> LFRAL;> AKCVSYGVAQIKAPALHSQGYTGSNVKVAILGTGIDSSHPDLNVAGGASFVPSETNPFQDNSSHGTHIAGTVLAVAPSASLYAVKVLGADGSGQASWVINGIEWAIANNMDVINMSLGSPSGSAALKAAVDKAVASGVVVVAAAGNSGTSGSSSTVTYPAKYPSVIAVGAVDSSNQRAPFSSVGPELDVMAPGVSICSTLPGGKYGALSGTSMASPHVAGAAALILSKHPNWTNTQVRSSLENTATKLGDSFYYGKGLINVEAAAQ

We describe the design, kinetic properties, and structures of engineered subtilisin proteases that degrade the active form of RAS by cleaving a conserved sequence in switch 2. The engineering process to develop specificity for the RAS sequence QEEYSAM involved extensive modification of the Bacillus protease, subtilisin BPN’16–24, a canonical serine protease in which the scissile peptide bond is attacked by a nucleophilic serine (S221). The nucleophilicity of S221 results from its interactions with the catalytic histidine (H64) and aspartic acid (D32) that together form a charge relay system. To generate high specificity for the RAS target sequence, the active site was modified to be dependent on a cofactor (imidazole or nitrite) and protease sub-sites were engineered to create a linkage between substrate and cofactor binding.

Based on this analysis, as well as earlier engineering work, we designed mutations in the catalytic region, the S1 pocket, and the S4 pocket to create a nitrite-dependent (D32G) protease and an imidazole-dependent (H64G) protease. These are denoted Protease1(N) and Protease1(I), respectively. The structure shows the enzyme complexed with a cognate peptide (LYRAL) and azide bound in the position normally occupied by the catalytic D32. The substrate-binding pockets and the azide binding site form an interconnected network. To understand the structural basis for specificity and cofactor activation, we determined crystal structures of RASProtease(I) alone, in complex with YSAM and QEEYSAM product peptides, and with imidazole. We compared these structures with the crystal structure of Protease1(N) in complex with a peptide corresponding to its sequence specificity (LFRAL, right). Overall the structures are very similar, with an RMSD between Cα carbons of 0.17 Å. The structures also provide insight into the structural basis for cofactor activation by both nitrite in Protease1(N) and imidazole in RASProtease(I). In both cases, a catalytic amino acid is mutated to Gly and the vacated space is occupied by a network of conserved water molecules in the absence of the cognate cofactor. Nitrite was modeled into the solvent network of the Protease1(N) structure (replacing HOH 54) such that it supplies the critical H-bond to the catalytic H64 and is coordinated to N33 and three conserved waters (23, 302, and 382).> SNPTTFSVEAIAAYTPVALIRLLNASGPLQPGHRVDIADARSIYTVGAAASAARARANHNANTIRRTAMFAETDPMTWLRPTVGLRRTFNPR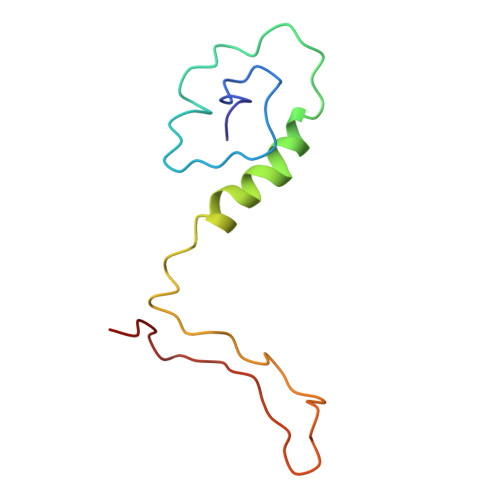II> MIERYVEFVGEHEIDAIFKYAEKLKDLSILHVNSTAAGGGVAEILHRLVPLMRELGLNAEWKVIRGSQDFFTVTKSFHNALQTGKGEIPDEYFKIYDEWQEINAGEIPLDYDVVFIHDPQPAGLVKYRKKGT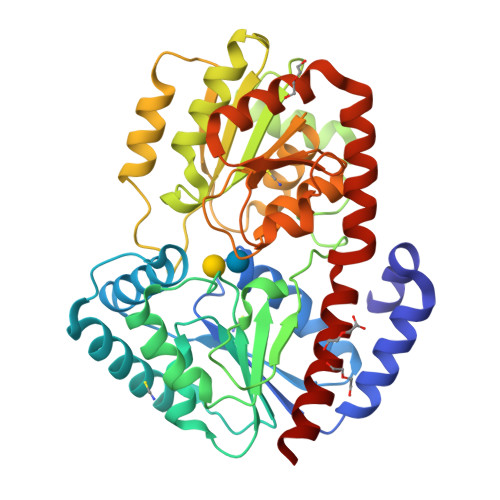WIWRCHIDISNPHPKVWGFLRGYISKYDGMIVSIPEFARDDLDIPQIAIPPSIDPLSPKNMPLPQTTVDRIVDKFGVDRERPIILQVSRYDRAKDPVGVIESFRLAKRHVPDAQLVYLGSPATDDPEGEVVYRETVEAARGEKDVHLLMLPPNSHVEVNAFQRAATVVMQKSIKEGFGLTVSEALWKRKPVIGGNTGGIRIQVINGVTGFLVDSPKAAAYYLVYLLKNKKVREEMGEAGRDHVRRNFLITQQLRRYLMAILYLTKRHA> MKTEWPELVGKSVEEAKKVILQDKPAAQIIVLPVGTIVTAEYRIDRVRLFVDRLDNIAQVPRV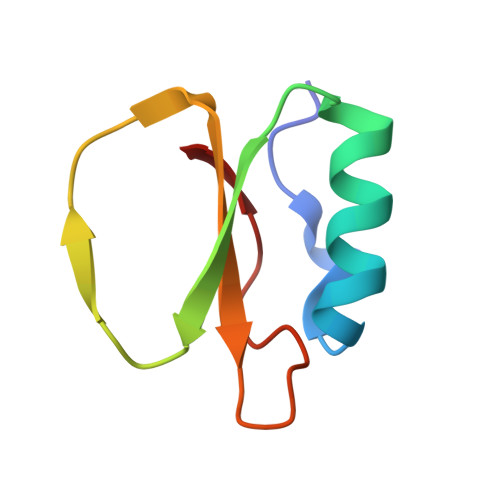G>GSHMILRPSMKLVKFRKGDSVGLRLAGGNDVGIFVAGVLEDSPAAKEGLEEGDQILRVNNVDFTNIIREEAVLFLLDLPKGEEVTILAQKKKDVYRRIVESDVGDSFYIRTHFEYEKESPYGLSFNKGEVFRVVDTLYNGKLGSWLAIRIGKNHKEVERGIIPNKNRAEQLASVQYTLPKTAGGDRADFWRFRGLRSSKRNLRKSREDLSAQPVQTKFPAYERVVLREAGFLRPVTIFGPIADVAREKLAREEPDIYQIAKSEPRDAGTDQRSSGI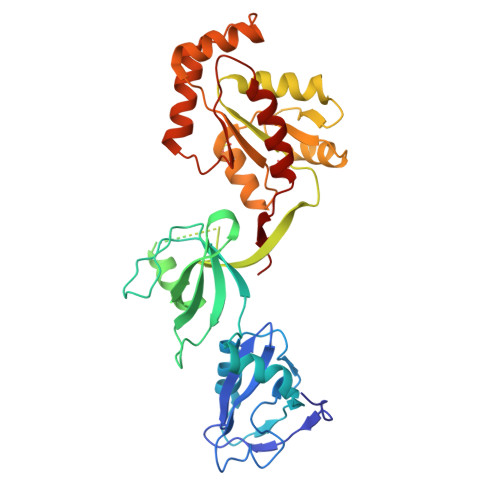IRLHTIKQIIDQDKHALLDVTPNAVDRLNYAQWYPIVVFLNPDSKQGVKTMRMRLCPESRKSARKLYERSHKLRKNNHHLFTTTINLNSMNDGWYGALKEAIQQQQNQLVWVSEG[4x]> ASTFSGVQSLPKFEIHDVRDDPAEGTMTRVAVDGKLLLISQYPQLGPRKVDPNDLSPQFDADRRISVRLRHVDLAYLVGVCKERVPRHRMETKAYTLDFEKSAQGYHLHGKVHRVASQRMEDWSVKFDNHFAVTLEHFLE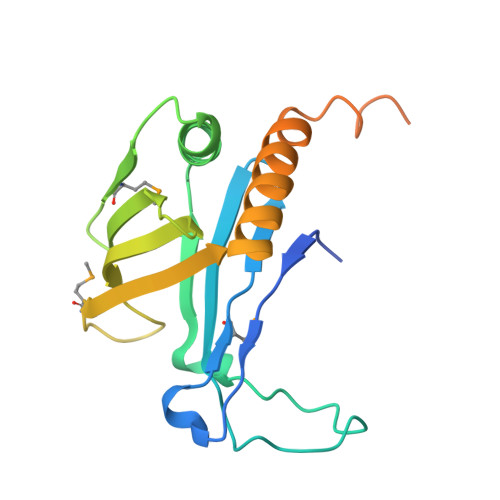SALDESFGFRQHYATRAAEGGEKIAATSSAEGGARRKRSVSDTSRYH> CCAUCCUCUACAGGCG;> 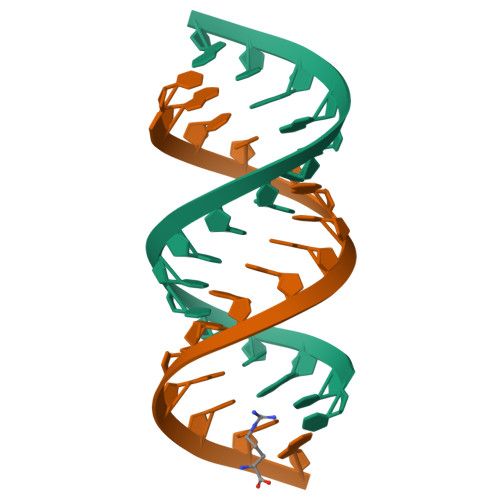CGCCUGUAGAGGAUGG> TQNSLSTSLQRLSSGLRINSAKDDAAGLAISDRMTAQIKGLTQAQRNANDGISLAQTAEGALGEISNNLQRIRELAVQASNGTNTQTDRDALQAEVTQLQSEIQRVAEQTSFNGQKLLDGSFNGVQFQIGANAGETIGVSKIMNAQ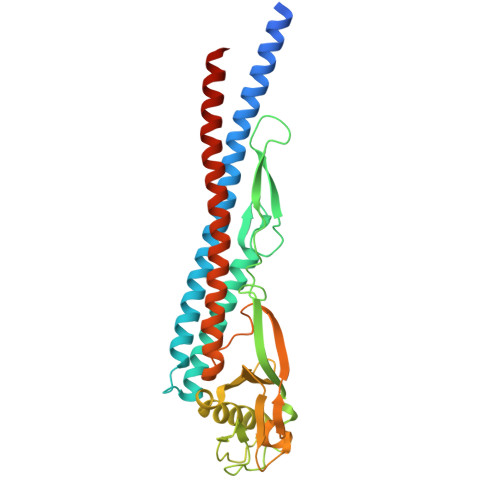TASLGGSLTRTTSTIDATDLTKYDTAMAAGDLTINGVDVGKIDAASTAQERAAQLTEAINRVSSQTNVGASYDKTTGQVTLTSNAAIAVAGAANDATVAGWANNATTGTATTTTGINSLTVSSFTNAQQTITQIDNALKDINTARADLGAVQNRFTSTVANLQSMTENLSSALEHHHHHH>MTKNKMEAKIDELINNDPVWSSQNESLISKPYNHILLKPGKNFRLNLIVQINRVMNLPKDQLAIVSQIVELLHNSSLLIDDIEDNAPLRRG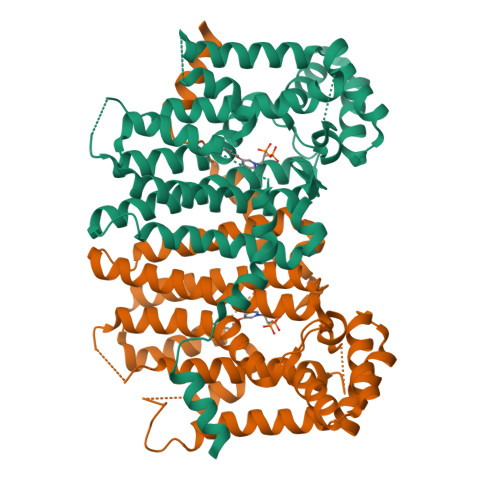QTTSHLIFGVPSTINTANYMYFRAMQLVSQLTTKEPLYHNLITIFNEELINLHRGQGLDIYWRDFLPEIIPTQEMYLNMVMNKTGGLFRLTLRLMEALSPSSHHGHSLVPFINLLGIIYQIRDDYLNLKDFQMSSEKGFAEDITEGKLSFPIVHALNFTKTKGQTEQHNEILRILLLRTSDKDIKLKLIQILEFDTNSLAYTKNFINQLVNMIKNDNENKYLPDLASHSDTATNLHDELLYIIDHLSEL[2x]>[2x]SMTSHSWLCDGRLLCLHDPSNKNNWKIFRECWKQGQPVLVSGVHKKLKSELWKPEAFSQEFGDQDVDLVNCRNCAIISDVKVRDFWDGFEIICKRLRSEDGQPMVLKLKDWPPGEDFRDMMPTRFEDLMENLPLPEYTKRDGRLNLASRLPSYFVRPDLGPKMYNAYGLITAEDRRVGTTNLHLDVSDAVNVMVYVGI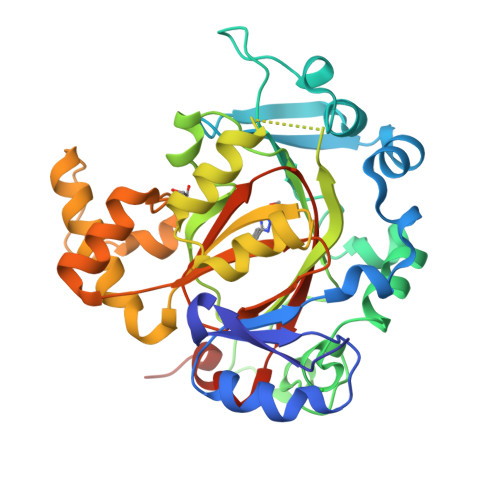PIGEGAHDEEVLKTIDEGDADEVTKQRIHDGKEKPGALWHIYAAKDAEKIRELLRKVGEEQGQENPPDHDPIHDQSWYLDQTLRKRLYEEYGVQGWAIVQFLGDAVFIPAGAPHQVHNLYSCIKVAEDFVSPEHVKHCFRLTQEFRHLSNTHT>[12x]MERNHWNEKSSGAKRSRERDLTLSTIRSILAADERLRIKASSYLGVGRGVDDEAVIDIFPTGQTMSFLRLLHGFLGTCRGQSMHQVLRDPCVLRKQLLYGVCKTLFDTITVRRVAEEWKLHAALFPYRALDEEDLEQYLLVWSASLRQSVQTGVLGALRDILYQYADNDDYGLYVDWCVTVGLVPLLDVKTKPSEAAERAQFVRAAVQRATETHPLAQDLLQANLALLLQVAERLGAVRVANAPEVRVFKKVRSERLEAQLRGKHIRLYVAAEPLAYERDKLLFTTPVAHLHEEILRYDGLCRHQKICQLLNTFPVKVVTASRHELNCKKLVEMMEQHDRGSDAKKSIMKFLLNVSDSKSRIGIEDSVESFLQDLTPSLVDQNRLLPARGPGGPGVVGPGGAVVGGPAGHVGLLPPPPGPAAPERDIRDLFKKQVIKCLEEQIQSQVDEIQDLRTLNQTWENRVRELRDLLTRYASRREDSMSLGARDAELYHLPVLEAVRKARDAAPFRPLAVEDNRLVANSFFSQFVPGTESLERFLTQLWENEYFRTFRLRRLVTHQGAEEAIVYSNYTVERVTLPYLCHILALGTLDPVPEAYLQLSFGEIVAAAYDDSKFCRYVELICSREKARRRQMSREAAGGVPERGTASSGGPGTLERSAPRRLITADEERRGPERVGRFRNGGPDDPRRAGGPYGFH

Here we present high-resolution structures of the A- and B-capsids and in-situ portals of human cytomegalovirus. The portal proteins are believed to orchestrate nucleation of the procapsid through the formation of a portal–scaffold complex, which facilitates procapsid assembly. During the maturation process, the disassociated scaffold proteins are expelled as the viral DNA is pumped into the capsid through the portal located at a unique vertex of the icosahedral capsid. All three capsids possess a mature icosahedral shell and are distinguishable by the inner capsid material: (1) C-capsids are filled with viral DNA; (2) A-capsids appear empty and are assumed to be products of aborted viral genome packaging; and (3) B-capsids have a featureless inner core consisting of scaffold proteins, likely generated by an unsuccessful initiation of DNA packaging.

Thus, the portals in B- and A-capsids represent to some extent the pre-DNA-packaging and the post-DNA-released states, respectively. Using high-resolution C12 portal reconstruction of the A-/B-capsids, we built the atomic model for the main body part of the portal protein pUL104, and showed that it consists of the wing (residues 52–90, 168–193 and 239–286), crown (residues 91–167, 194–238 and 570–647), stem (residues 287–314 and 528–551), clip (residues 315–322 and 485–527) and β-hairpin (residues 552–569) domains. The main body of the DNA-devoid portal has a hollow central channel with three constricted regions harboring interior diameters of 30, 33, and 73 Å, respectively. Furthermore, the portal main body of the A-/B-capsid locates ~20 Å inward; in contrast, each of the 12 monomers from the portal main body of the DNA-filled capsid rotates inward. As a result, whereas the crown domain shows the greatest movement (up to 7.9 Å) toward the central channel, we noted a gradual decrease in the movements of the β-hairpin domain (with the tip sliding by 5.3 Å), wing domain (an RMSD of 2.10 Å) and stem/clip domains (RMSDs of 1.28 Å/1.88 Å). The portals from the A- and B-capsid resemble each other and are arranged in a symmetry-mismatch fashion different from that of the virion: a C5 10-helix anchor, a C5 portal turret, and a C12 portal main body. A portal structural comparison of the DNA-free and DNA-filled capsids shows that the scaffold fragment binding cavity of the portal is closed off in the virion capsid, suggesting that dissociation of the scaffold fragments from the portal is necessary for the required portal conformational changes during DNA translocation. Given that the portal in the A-capsid, which somewhat represents the post-release state, is identical to that in the B-capsid both conformationally and positionally, we believe that inner capsid pressure generated by the packaged DNA causes the conformational changes of the portal.(2~{R})-~{N}-[4-ethanoyl-5-[4-(2-oxidanylidenepyrrolidin-1-yl)phenyl]-1,3-thiazol-2-yl]piperazine-2-carboxamide | C20 H23 N5 O3 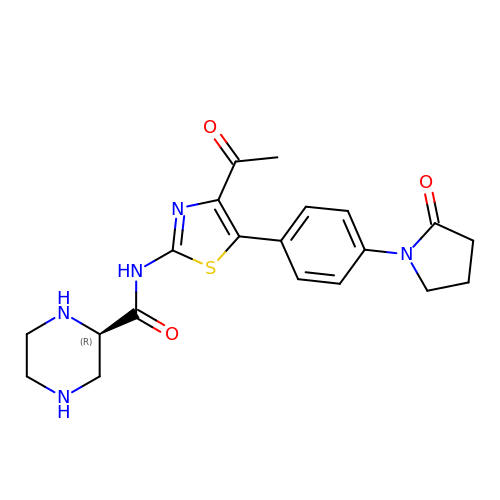S | OKMNIGWEMMUEAF-OAHLLOKOSA-N>MAKVFQWFGSNESGAEFGSQNLPGVEGKDYIWPDPNTIDTLISKGMNIFRVPFMME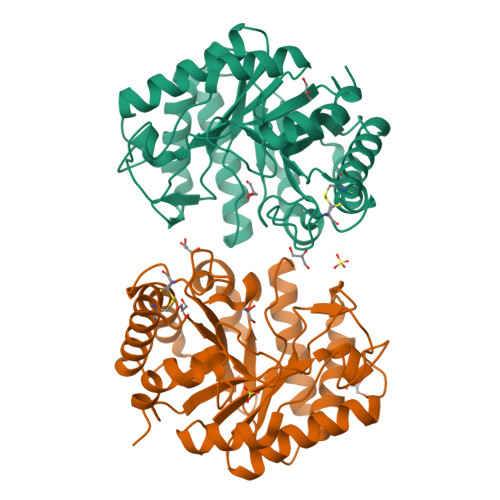RLVPNSMTGSPDPNYLADLIATVNAITQKGAYAVVDPHNYGRYYNSIISSPSDFQTFWKTVASQFASNPLVIFDTNNAYHDMDQTLVLNLNQAAIDGIRSAGATSQYIFVEGNSWTGAWTWTNVNDNMKSLTDPSDKIIYEMHQYLDSDGSGTSATCVSSTIGQERITSATQWLRANGKKGIIGEFAGGANDVCETAITGMLDYMAQNTDVWTGAIWWAAGPWWGDYIFSMEPDNGIAYQQILPILTPYL[2x]>TELTVDQQTLLDYIMDSYSKQRMPQEITNKILKEEFSAEENFLILTEMATSHVQILVEFTKRLPGFQTLDHEDQIALLKGSAVEAMFLRSAEIFNKKLPAGHADLLEERIRKSGISDEYITPMFSFYKSVGELKMTQEEYALL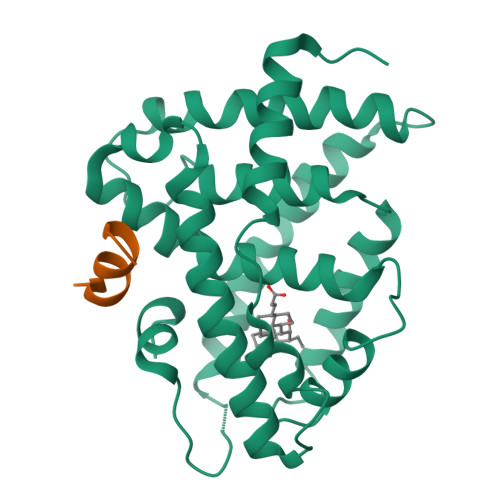TAIVILSPDRQYIKDREAVEKLQEPLLDVLQKLCKIYQPENPQHFACLLGRLTELRTFNHHHAEMLMSWRVNDHKFTPLLCEIWDV[2x];>[3x]ENALLRYLLDKD WaaP, a cytoplasmic soluble protein, phosphorylates the first heptose sugar of LPS inner core, which appears to be required for subsequent core phosphorylation steps. Here, we report the first X-ray crystallographic structure of P. aeruginosa WaaP, expressed in Escherichia coli, which revealed a very tight and novel complexation with E. coli acylated acyl-carrier protein (acyl-ACP). However, here we discovered that acyl-ACP acts as a very tightly bound cofactor necessary for the production and stability of active WaaP kinase, uncovering a new function for acyl-ACP. The catalytic core of the protein kinase family was mostly conserved and demonstrated to be essential for WaaP cellular function, suggesting a conserved EPK-like mechanism of ATP dependent phosphotransfer.

The final crystal structure contained a 1:1 complex of P. aeruginosa WaaP and E. coli acyl-ACP. The structural topology of the WaaP kinase consisted of a 6-stranded β-sheet NH-terminal lobe (1-118) flanked by two α-helices (19-24 and 73-89) with strong structural homology to eukaryotic protein kinase (EPK) family members, as expected from primary sequence analysis, and a predominantly helical COOH-terminal lobe (119-263). The COOH-terminal lobe was further divided into two sub-domains: the first sub-domain (I) (119-218) had structural homology to EPKs and the second sub-domain (II) (218-263) was composed of a novel arrangement of three helices, forming a channel through which a tube of electron density (approximately 20 Å long and 7 Å wide) extended into the COOH-terminal sub-domain I, ending under the kinase active site pocket. The density was consistent with a palmitoyl group (C16:0) on ACP. Weaker density matching a phosphopentatheine group extended from S36 in E. coli ACP that positioned the lipid palmitoyl group in the hydrophobic channel of P. aeruginosa WaaP. Structurally, the EPK-family residues required for ATP binding and phosphotransferase were mostly present, however important differences were observed that placed WaaP in the eukaryotic protein kinase-like (ELK) family. Differences from classic EPK structure elements included the novel COOH-terminal sub-domain, a modified Mg2+ binding activation loop where histidine (H168 in WaaP) coordinated to the second Mg2+ ion in place of a conserved asparagine residue (N171 in protein kinase A), and a shortened, structured WaaP activation loop lacking EPK regulatory elements. The WaaP/acyl-ACP interface was composed of two discreet interactions: a ~645 Å2 hydrophilic PPI and the insertion of the lipid chain of acyl-ACP into a ~680 Å2 hydrophobic invagination in the COOH-terminal lobe of WaaP. The hydrophilic PPI was formed by interactions between the negatively charged surface of ACP (residues D35, E41, E47, E48, E53 and D56) with a positively charged surface on WaaP (residues K140, R141, R221, R222, R226, R229 and R237).

> MRLVLEEPFKRLWNGRDPFEAVEALQGKVYRELEGRRTLRTEVDGRGYFVKIHRGIGWGEIAKNLLTAKLPVLGARQEWQAIRRLHEAGVATMTAVAYGERGSDPARQHSFIVTEELAPTVDLEVFSQDWRERPPPPRLKRALVEAVARMVGDMHRAGVNHRDCYICHFLLHTDKPVSADDFRLSVIDLHRAQTRDATPKRWRNKDLAALYFSALDIGLTRRDKLRFLRTYFRRPLREILRDEAGLLAWMERKAEKLYE;> TIEERVKKIIGEQLGVKQEEVTNNASFVEDLGADSLDTVELVMALEEEFDTEIPDEEAEKITTVQAAIDYIN> MIYSRSKLPSEGEILIATVKQVFDYGSYVSLDEYGGLQAFLPWSEVSSKWVKNIRDVLKENRKVIVKVIRVDRRKGTVDVSLKKVTDDERRKKNLQWKKIQRLDKILELVSQKLKLSEKDAWEQVAWKLEAKYGDPITAIEKAVKEGEKILIDAGVPEIWVKPLLEEA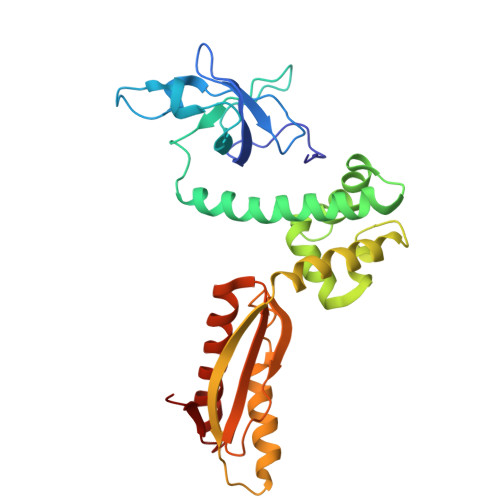SKHAEERKVKMSGLITVRTNEPLGVEKIKEVISKALENIEQDYESLLNIKIYTIGAPRYRVDVVGTNPKEASEALNQIISNLIKIGKEENVDISVVKK> MKKARRSPSRRKGARLWY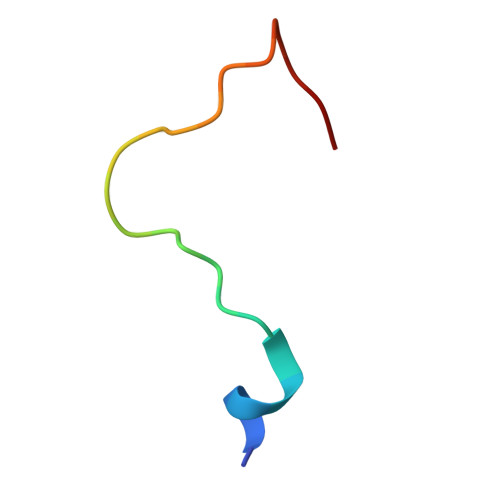VGGSQF>[3x]MPMFIVNTNVPRASVPDGFLSELTQQLAQATGKPPQYIAVHVVPDQ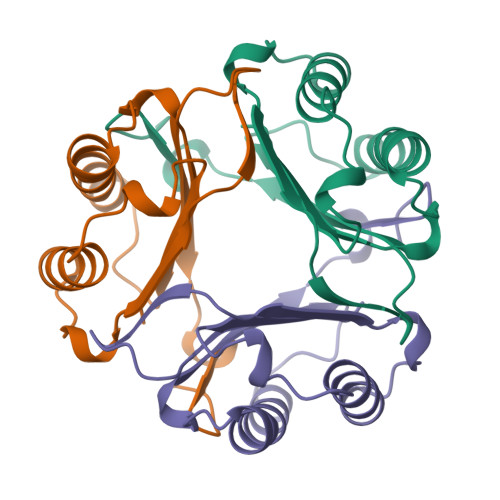LMAFGGSSEPCALCSLHSIGKIGGAQNRSYSKLLCGLLAERLRISPDRVYINYYDMNAANVGWNNSTFA> DLTVKEKEELIEEWQPEPLVPPVPKDHPALNYNIVSGPPSHKTVVNGKECINFASFNFLGLLDNPRVKAAALASLKKYGVGTCGPRGFYGTFDVHLDLEDRLAKFMKTEEAIIYSYGFATIASAIPAYSKRGDIVFVDRAACFAIQKGLQAS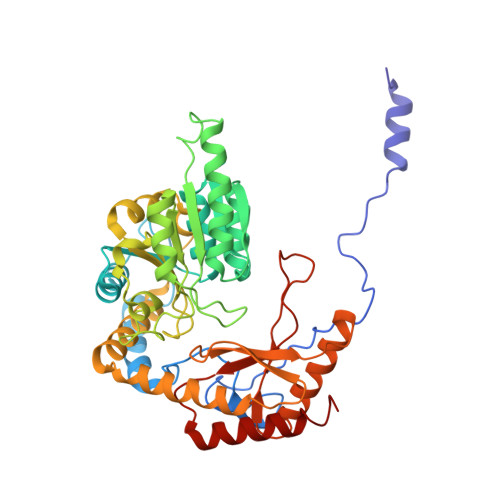RSDIKLFKHNDMADLERLLKEQEIEDQKNPRKARVTRRFIVVEGLYMNTGTICPLPELVKLKYKYKARIFLEESLSFGVLGEHGRGVTEHYGINIDDIDLISANMENALASIGGFCCGRSFVIDHQRLSGQGYCFSASLPPLLAAAAIEALNIMEENPGIFAVLKEKCGQIHKALQGISGLKVVGESLSPAFHLQLEESTGSREQDVRLLQEIVDQCMNRSIALTQARYLEKEEKCLPPPSIRVVVTVEQTEEELERAASTIKEVAQAVLL>[2x]MWLLALCLVGLAGAQRGGGGPGGGAPGGPGLGLGSLGEERFPVVNTAYGRVRGVRRELNNEILGPVVQFLGVPYATPPLGARRFQPPEAPASWPGVRNATTLPPACPQNLHGALPAIMLPVWFTDNLEAAATYVQNQSEDCLYLNLYVPTEDGPLTKKRDEATLNPPDTDIRDPGKKPVMLFLHGGSYMEGTGNMFDGSVLAAYGNVIVATLNYRLGVLGFLSTGDQAAKG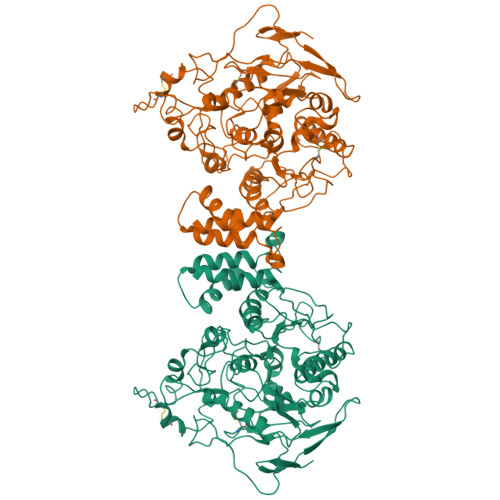NYGLLDQIQALRWLSENIAHFGGDPERITIFGSGAGASCVNLLILSHHSEGLFQKAIAQSGTAISSWSVNYQPLKYTRLLAAKVGCDREDSAEAVECLRRKPSRELVDQDVQPARYHIAFGPVVDGDVVPDDPEILMQQGEFLNYDMLIGVNQGEGLKFVEDSAESEDGVSASAFDFTVSNFVDNLYGYPEGKDVLRETIKFMYTDWADRDNGEMRRKTLLALFTDHQWVAPAVATAKLHADYQSPVYFYTFYHHCQAEGRPEWADAAHGDELPYVFGVPMVGATDLFPCNFSKNDVMLSAVVMTYWTNFAKTGDPNQPVPQDTKFIHTKPNRFEEVVWSKFNSKEKQYLHIGLKPRVRDNYRANKVAFWLELVPHLHNLHTELFTTTTRLPPYATRWPPRPPAGAPGTRRPPPPATLPPEPEPEPGPRAYDRFPGDSRDYSTELSVTVAVGASLLFLNILAFAALYYKRDRRQELRCRRLSPPGGSGSGVPGGGPLLPAAGRELPPEEELVSLQLKRGGGVGADPAEALRPACPPDYTLALRRAPDDVPLLAPGALTLLPSGLGPPPPPPPPSLHPFGPFPPPPPTATSHNNTLPHPHSTTRV>MSNSAETDVLIVGAGPAGAMSATLLASLGIRSLMINRWRSTSPGPRSHIINQRTMEILRDIGLEESAKSLAVPKEYMGEHVYATSLAGEEFGRIPAWASHPQAHAEHELASPSRY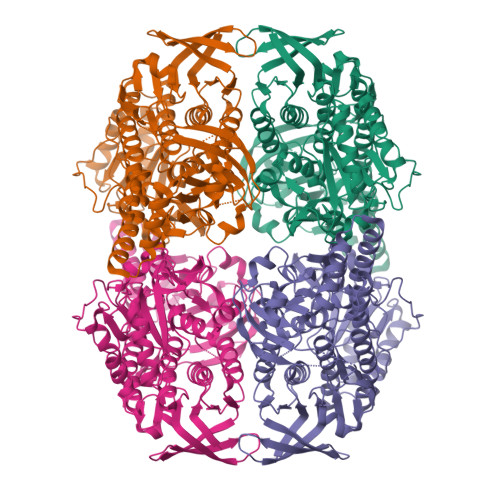CDLPQLYFEPMVVSEAALRGADVRFLTEYLGHVEDQDGVTARLLDHVSGAEYEVRAKYIIGADGAHSLVAQNAGLPFEGQMGIGDSGSINIEFSADLSSLCEHRKGDMYWMFRAGSGINGVGVAALRMIRPWNKWICVWGYEKSKGTPEITKEEAKKIIHEIIGTDEIPVEVGPISTWTINQQYAVRNTSGRVFCMGDAVHRHTPMGGLGLNTSVQDAYNLAWKLALVLKGQAAPTLLDSYDAERSPVAKQIVERAFKSLSTFPPVFEALSLPPAPTESEMAEALVRLKDASEEGAKRRAALRKAMDATIIGLGGGHGVELNQRYVSRAVFPDGTPDPGFVRDQEFFYQASTRPGAHLPHVWLTENQRRISTLDLCGKGRFTLLTGLSGAAWKHEAEQVSQSLGIELKVCVIGPGQEFVDTYGEYAKISEIGESGALLVRPDMFIAFRAKDASREGLEQLNVAVKSILGRA[4x]> MQHYLHIRPAPSDNLPLVDLIEHPDPIFDPKEKDLNETLLRSLLGGHYDPGFMATSPPEDRPGGGGGAAGGAEDLAELDQLLRQRPSGAMPSEIKGLEFSEGLAQGKKQRLSKKLRRKLQMWLWSQTFCPVLYAWNDLGSRFWPRYVKVGSCFSKRSCSVPEGMVCKPSKSVHLTVLRWRCQRRGGQRCGWIPIQYPIISECKCSC;> QAKHKQRKRLKSSCKRHPLYVDFSDVGWNDWIVAPPGYH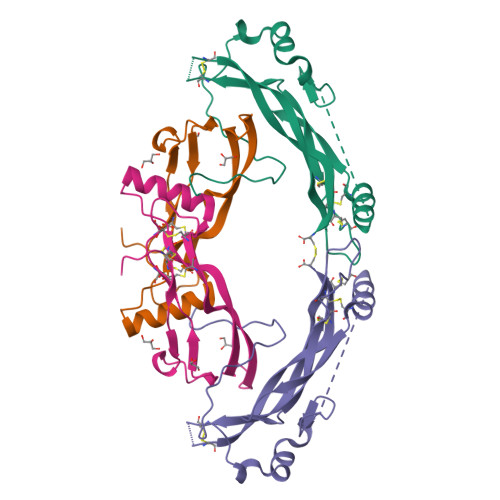AFYCHGECPFPLADHLNSTNHAIVQTLVNSVNSKIPKACCVPTELSAISMLYLDENEKVVLKNYQDMVVEGCGCR> MKQVKIMFLMTMFLGIGLLFFSENAEAAITSNEIGTHDGYDYEFWKDSGGSGSMTLNSGGTFSAQWSNVNNILFRKGKKFDETQTHQQIGNMSINYGATYNPNGNSYLTVYGWTVDPLVEFYIVDSWGTWRPPGGTPKGTINVDGGTYQIYETTRYNQPSIKGTATFQQYWSVRTSKRTSGTISVSEHFRAWESL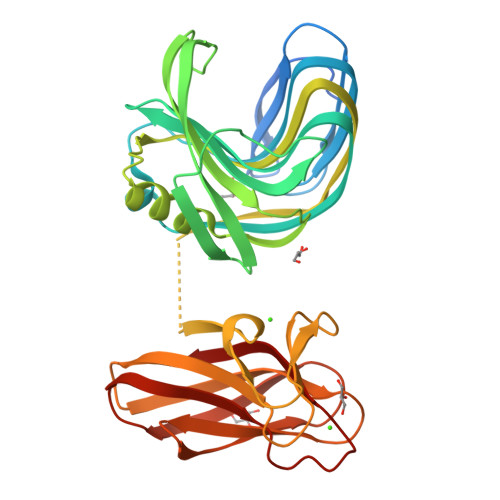GMNMGNMYEVALTVEGYQSSGSANVYSNTLTIGGQSGGEQATRVEAESMTKGGPYTSNITSPFNGVALYANGDNVSFNHSFTKANSSFSLRGASNNSNMARVDLRIGGQNRGTFYFGDQYPAVYTINNINHGIGNQLVELIVTADDGTWDAYLDYLEIR> MRGSHHHHHHGSAEKQERVQHLHDIRDLHRYYSSESFEYSNVSGKVENYNGSNVVRFNPQNHQLFLLGKDKEQYKEGLQGQNVFVVQELIDPNGRLSTVGGVTKKNNKTSETNTPLFVNKVNGEDLDASIDSFLIQKEEISLKELDFKIRQQLVNNYGLYKGTSKYGKIIINLKDENKVEIDLGDKLQFERMGDVLNSKDIRGISVTINQI;> MRGSHHHHHHGSAEKQERVQHLHDIRDLHRYYSSESFEYSNVSGKVENYNGSNVVRFNPKDQNHQLFLLGKDKEQYKEGLQGQNVFVVQELIDPNGRLSTV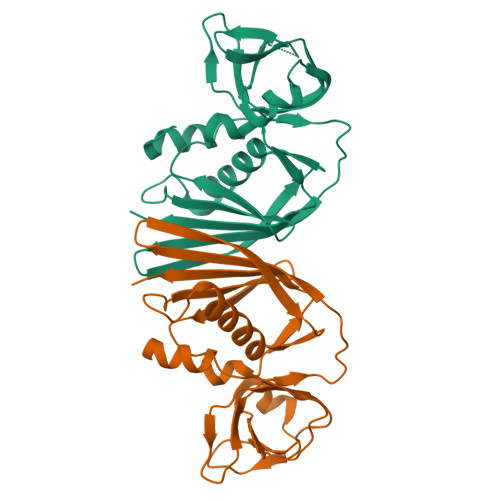GGVTKKNNKTSETNTPLFVNKVNGEDLDASIDSFLIQKEEISLKELDFKIRQQLVNNYGLYKGTSKYGKIIINLKDENKVEIDLGDKLQFERMGDVLNSKDIRGISVTINQI>[8x]GSQIHVDTMKVINDPIHGHIELHPLLVRIIDTPQFQRLRYIKQLGGGYYVFPGASHNRFEHSLGVGYLAGCLVHALGEKQPELQISERDVLCVQIAGLCHDLGHGPFSAMFDGRFIPLARPEVKWTHEQGSVMMFEHLINSNGIKPVMEQYGLIPEEDICFIKEQIVGPLESPVEDSLWPYKGRPENKSFLYEIVSNKRNGIDVDKWDYFARDCHHLGIQNNFDYKRFIKFARVCEVDNELRICARDKEVGNLYDMFHTRNSLHRRAYQHKVGNIIDTMITDAFLKADDYIEITGAGGKKYRISTAIDDMEAYTKLTDNIFLEILYSTDPKLKDAREILKQIEYRNLFKYVGETQPTGQIKIKREDYESLPKEVASAKPKVLLDVKLKAEDFIVDVINM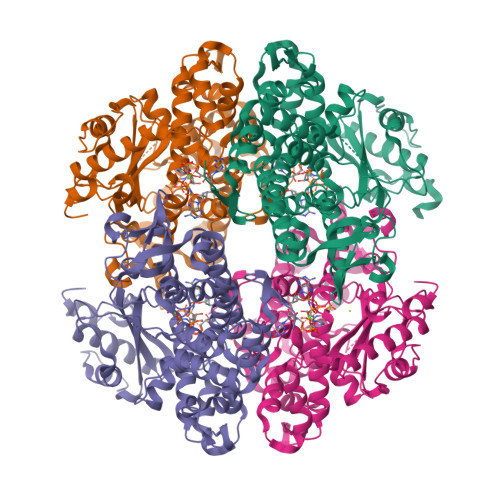DYGMQEKNPIDHVSFYCKTAPNRAIRITKNQVSQLLPEKFAEQLIRVYCKKVDRKSLYAARQYFVQWCADRNFTKPQDGDVIAPLITPQKKEWNDSTSVQNPTRLREASKSRVQLFKDDPM> MAVTYNPQTKQFHLRAGKASYVMQLFRSGYLAHIYWGKAVRDVRGERRFSRLDRAFSPNPDPSDRTFSLDTLPQEYPAYGNTDFRSPAYQVQLENGSTVTDLRYKTHRIYKGKPRLNGLPATYVEHEQEAETLEIVLGDALIGLEVTLQYTAYEKWNVITRAARFENKGGERLKLLRALSMSVDFPTADYDWIHLPGAWGRERWIERRPLVTGVQAAESRRGASSHQQNPFIALVAKNADEHQGEVYGFSFVYSGNFLAQVEVDQFHTARVSMGINPFDFTWLLQPGESFQTPEVVMVYSDQGLNGMSQTYHELYRTRLARGAFRDRERPILINNWEATYFDFNEEKLVNIAKTEAELGIELFVLDDGWFGKRDDDRRSLGDWIVNRRKLPNGLDGLAKQVNELGMQFGLWVEPEMVSPNSELYRKHPDWCLHVPNRPRSEGRNQLVLDYSREDVCDYIIETISNVLASAPITYVKWDMNRHMTEIGSSALPPERQRETAHRYMLGLYRVMDEMTSRFPHILFESCSGGGGRFDPGMLYYMPQTWTSDNTDAVSRLKIQYGTSLVYPISAMGAHVSAVPNHQVGRVASLKARGHVAMSGNFGYELDITKLTETEKQMIKQQVAFYKDVRRLVQFGTFYRLLSPFEGNEAAWMFVSADRSEALVAYFRVLAEAN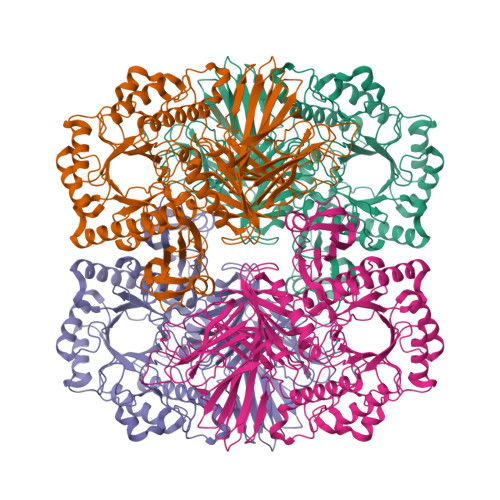APLSYLRLKGLDPNQDYEIEGLGVYGGDELMYAGVALPYRSGDFISMMWRLKAVQQ>SQKVEKTVIKNETGTISISQLNKNVWVHTELGSFNGEAVPSNGLVLNTSKGLVLVDSSWDDKLTKELIEMVEKKFQKRVTDVIITHAHADRIGGIKTLKERGIKAHSTALTAELAKKNGYEEPLGDLQTVTNLKFGNMKVETFYPGKGHTEDNIVVWLPQYNILVGGCLVKSTSAKDLGNVADAYVNEWSTSIENVLKRYRNINAVVPGHGEVGDKG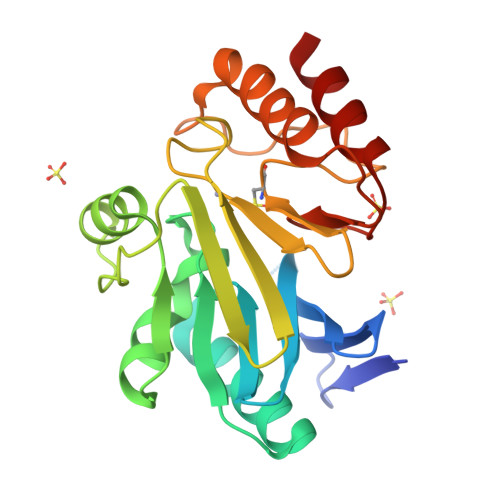LLLHTLDLLK[2x]> GSHMLEDPLRVSPMIREFVQSIDDREWQTQLFALLQKQTYNQVEVDLFELMCKVLDQNLFSQVDWA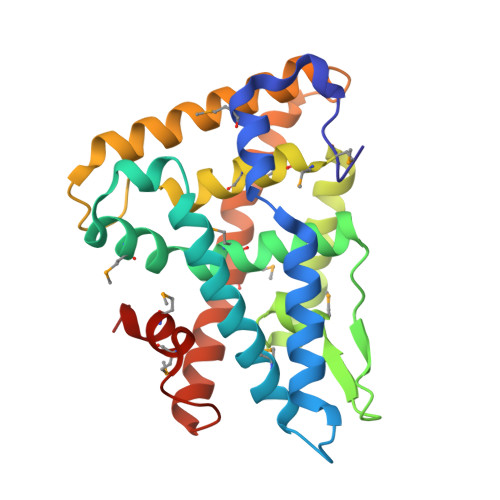RNTVFFKDLKVDDQMKLLQHSWSDMLVLDHLHHRIHNGLPDETQLNNGQVFNLMSLGLLGVPQLGDYFNELQNKLQDLKFDMGDYVCMKFLILLNPSVRGIVNRKTVSEGHDNVQAALLDYTLTCYPSVNDKFRGLVNILPEIHAMAVRGEDHLYTKHCAGSAPTQTLLMEMLHAKRKG6-{[(1R,3S)-3-phenylcyclopentyl]amino}pyridine-3-carboxamide | C17 H19 N3 O | 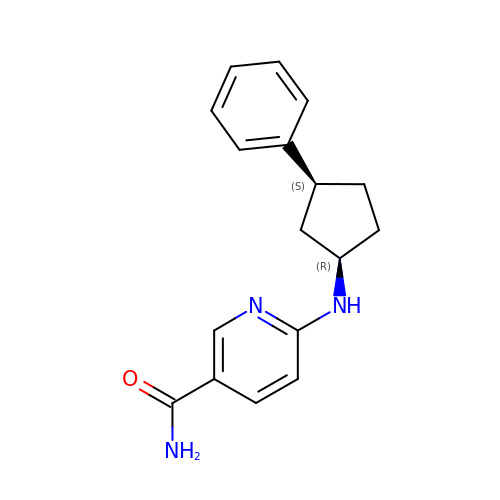JBSAILAEEJVXKB-DZGCQCFKSA-N(3~{R})-3-azanyl-4-[5-[4-(4-chloranylphenoxy)phenyl]-1,2,3,4-tetrazol-2-yl]butanoic acid | C17 H16 Cl N5 O3 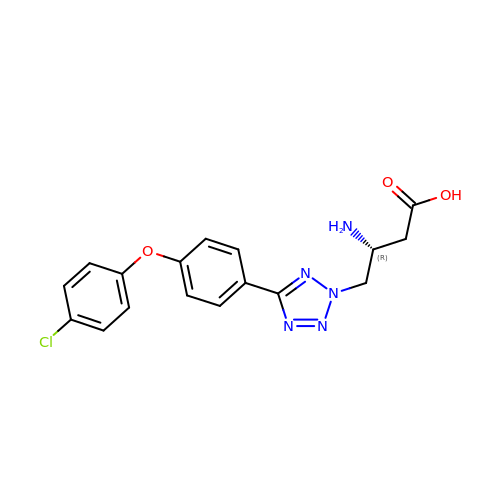| VSQILWJHLPJYGP-CYBMUJFWSA-N>[8x]GSEELLDLFNRQVTQEFTASQVYLSASIWFDQNDWEGMAAYMLAESAEEREHGLGFVDFANKRNIPIELQAVPAPVSCAEWSSPED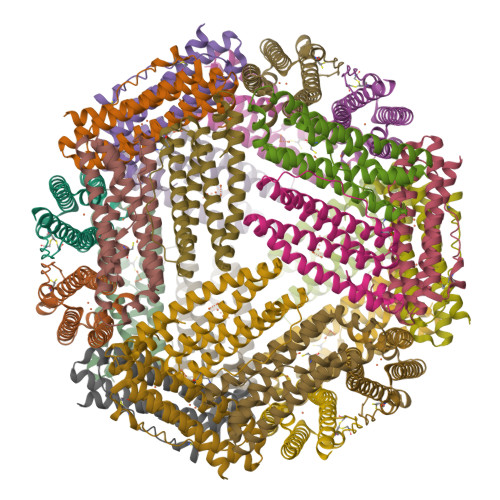VWQSILELEQANTRSLLNLAEAASTCHDFAVMAFLNPFHLQQVNAEDKIGSILAKVTDENRTPGLLRSLDVVSFLGPCLFRS>[3x]MKLPVREFDAVVIGAGGAGMRAALQISQSGQTCALLSKVFPTRSHTVSAQGGITVALGNTHEDNWEWHMYDTVKGSDYIGDQDAIEYMCKTGPEAILELEHMGLPFSRLDDGRIYQRPFGGQSKNFGGEQAARTAAAADRTGHALLHTLYQQNLKNHTTIFSEWYALDLVKNQDGAVVGCTALCIETGEVVYFKARATVLATGGAGRIYQSTTNAHINTGDGVGMAIRAGVPVQDMEMWQFHPTGIAGAGVLVTEGCRGEGGYLLNKHGERFMERYAPNAKDLAGRDVVARSIMIEIREGRGCDGPWGPHAKLKLDHLGKEVLESRLPGILELSRTFAHVDPVKEPIPVIPTCHYMMGGIPTKVTGQALTVNEKGEDVVVPGLFAVGEIACVSVHGANRLGGNSLLDLVVFGRAAGLHLQESIAEQGALRDASESDVEASLDRLNRWNNNRNGEDPVAIRKALQECMQHNFSVFREGDAMAKGLEQLKVIRERLKNARLDDTSSEFNTQRVECLELDNLMETAYATAVSANFRTESRGAHSRFDFPDRDDENWLCHSLYLPESESMTRRSVNMEPKLRPAFPPKIRTY;>[3x]MRLEFSIYRYNPDVDDAPRMQDYTLEADEGRDMMLLDALIQLKEKDPSLSFRRSCREGVCGSDGLNMNGKNGLACITPISALNQPGKKIVIRPLPGLPVIRDLVVDMGQFYAQYEKIKPYLLNNGQNPPAREHLQMPEQREKLDGLYECILCACCSTSCPSFWWNPDKFIGPAGLLAAYRFLIDSRDTETDSRLDGLSDAFSVFRCHSIMNCVSVCPKGLNPTRAIGHIKSMLLQRNA;>[3x]MIRNVKKQRPVNLDLQTIRFPITAIASILHRVSGVITFVAVGILLW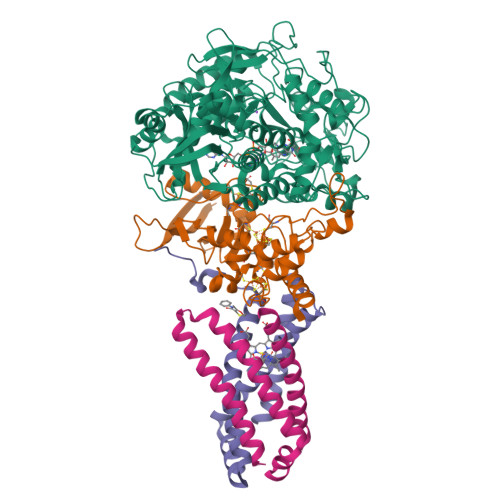LLGTSLSSPEGFEQASAIMGSFFVKFIMWGILTALAYMVVVGIRHMMMDFGYLEETFEAGKRSAKISFVITVVLSLLAGVLVW;>MVSNASALGRNGVHDFILVRATAIVLTLYIIYMVGFFATSGELTYEVWIGFFASAFTKVFTLLALFSILIHAWIGMWQVLTDYVKPLALRLMLQLVIVVALVVYVIYGFVVVWGV[3x]>[2x]PFATADIAEKMWAENYETTSPAPVLVAEGEQVTIPCTVMTHSWPMVSIRARFCRSHDGSDELILDAVKGHRLMNGLQYRLPYATWNFSQLHLGQIFSLTFNVSTDTAGMYECVLRNYSHGLIMQRFVILTQLETLSRPDEPCCTPALGRYSLGDQIWSPTPWRLRNHDCGMYRGFQRNYFYIGRADAEDCWKPACPDEEPDRCWTVIQRYRLPGD;>QQDLAPQQRAAPQQKRSSPSEGLCPPGHHISEDGRDCISCKYGQDYSTHWNDLLFCLRCTRCDSGEVELSPCTTTRNTVCQCEEGTFREEDSPEMCRKCRTGCPRGMVKVGDCTPWSDIECVHKESG[2x]

Here, we report the structural and biochemical characterization of the novel, non-canonical interaction between UL141 and TRAIL-R2, an interaction that has evolved to inhibit cell death mediated by TRAIL signaling and mute host defenses. Remarkably, UL141 displays no structural homology to TNF superfamily ligands, and instead utilizes its Ig-domain to bind with high affinity to the TRAIL death receptor. UL141 utilizes at least two distinct binding sites to selectively engage TRAIL death receptors and the NK cell activating ligand CD155. We have shown that cells infected with an HCMVΔUL141 mutant are more susceptible to killing by TRAIL, and that UL141 is both necessary and sufficient to retain both TRAIL receptors in the ER, thus preventing their cell surface expression.

The complex of HCMV UL141 (residues 30–279) bound to human TRAIL-R2 (residues 58–184, both numberings start from the initial methionine) was crystallized and the structure determined by single anomalous dispersion (SAD), using experimental phases derived from selenomethionine labeled protein expressed in Sf9 insect cells. The crystal structure was refined to a resolution of 2.1 Å with an R factor of 22.3% and an Rfree of 27.4%. One UL141 dimer binds two TRAIL-R2 monomers through non-crystallographic two-fold symmetry resulting in a heterotetrameric complex. Structural analysis revealed that UL141 interacts in a head-to-tail fashion to form a well-packed dimer that is stabilized primarily through polar interactions, such as hydrogen bonds and salt bridges, and several hydrophobic contacts, while burying a total surface area of 1423 Å2. The UL141 ectodomain exhibits an N-terminal immunoglobulin (Ig)-like domain, followed by an additional C-terminal β-sheet domain. In contrast to TRAIL binding to TRAIL-R2, which leads to head-to-head (180°) trimerization of the receptor, UL141 binds both TRAIL-R2 monomers diagonally across the entire UL141 ectodomain, resulting in an approximate rotation of both TRAIL-R2 monomers of 90° to each other. The high affinity interaction between UL141 and TRAIL-R2 correlates well with the large solvent-accessible surface area of the heterotetrameric complex in which 2694 Å2 are buried on the UL141 dimer (1347 Å2 per monomer) and 1351 Å2 are buried on each TRAIL-R2 monomer. CRD-1–3 span a length of 70 Å, and CRD-2 and CRD-3 form the major ligand-binding region in the UL141–TRAIL-R2 complex. The combined structural and mutational data suggest that contact patch 4 is specific and crucial for TRAIL ligand binding and that viral UL141 mimics this structural motif to specifically engage this TRAIL DR. In summary, patch 5 involves strong hydrophobic features important for the stability of complexes throughout the TNF/TNFR superfamily, and we postulate that UL141 has evolved to mimic this interaction in order to modulate this TRAIL DR.>MSLKGKRIGFGFTGSHCTYEEVMPHLEKLIAEGAEVRPVVSYTVQSTNTRFGEGAEWIKKIEEITGFKAINSIVGAEPLGPKIPLDCMVIAPLTGNSMSKFANAMTDSPVLMAAKATLRNGKPVVLAVSTNDALGLNGVNLMRLMATKNIYFVPFGQDAPEKKPNSMVARME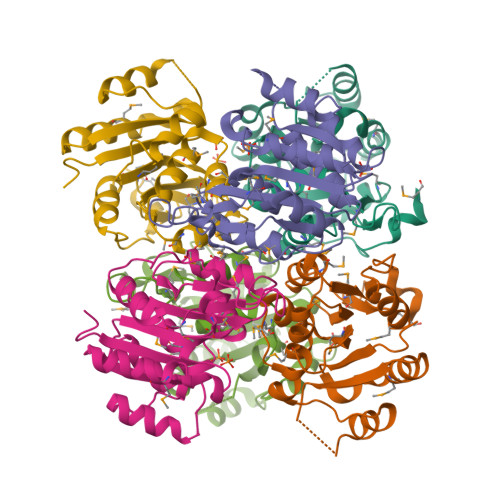LLEDTVLEALQGKQLQPVVVEKFRYMNLEHHHHHH[6x]>MAEIPKEMLRAQTNAILLNVLKQGDNYVYGIIKQVKEASNGEMELNEATLYTIFKRLEKDGIISSYWGDESQGGRRKYYRLTEIGHENMRLAFESWSRVDKIIENLEANKKSEAIKSRWSHPQFEK[2x]

We present a new class of ArMs featuring a genetically encoded noble‐metal‐binding site based on a non‐canonical thiophenol‐based amino acid, 4‐mercaptophenylalanine (pSHF), incorporated in the transcriptional regulator LmrR through stop codon suppression. Next, we investigated the incorporation of pSHF into Lactococcal multidrug resistance regulator (LmrR), which has been demonstrated to be a highly versatile protein scaffold for artificial enzyme design. We selected position V15 for incorporation, since this places pSHF inside the hydrophobic pocket at the dimer interface. Here, we report a new class of artificial metalloenzymes featuring a genetically encoded thiophenol for binding noble metals and the application of this design approach by the creation of an artificial gold enzyme that shows efficient catalysis of abiological hydroamination reactions.

After establishing the incorporation and position of the pSHF residues in LmrR using X‐ray crystallography, we aimed to establish the binding mode of the gold ions in LmrR_V15pSHF−Au. An X‐ray crystal structure at 2.50 Å resolution was obtained via co‐crystallisation with KAuCN2, which is more water‐soluble than Au(SMe2)Cl and has been used extensively for heavy atom phasing in protein X‐ray crystallography. The crystal structure and crystallographic Fourier maps revealed the presence of one gold ion, coordinating one of the two pSHF residues in the LmrR_V15pSHF dimer (Supporting Information section 9). The gold atom is associated with a strong peak in the anomalous difference Fourier map, unambiguously establishing its identity and position in the crystal structure. In addition to the sulphur of the pSHF residue, a hydroxyl ion or water molecule appears to serve as a coordinating ligand of the gold ion, establishing a linear two‐coordination arrangement that is typical for Au(I). The gold atom is surrounded by the side chains of Asn19, Lys22, Phe93, and Met89 at a minimal distance of 4–5 Å, establishing a second coordination sphere and restricting the solvent accessibility of the gold. No clear anomalous difference peak is present near the other pSHF residue, and the electron density of this residue appears distorted and weak compared to its counterpart in the dimer, indicative of substantial conformational disorder. Although it is possible that gold is also bound to this second pSHF residue, contributing to the observed disorder, the X‐ray data is insufficient to determine this conclusively. Aggregate formation of LmrR_V15pSHF−Au is avoided because the two thiophenolic residues are spatially separated in the protein dimer. Of these, we selected two positions for site‐saturation mutagenesis: A11, which showed a faster reaction upon substitution to leucine, and M89, which in the crystal structure is in close proximity of the pSHF‐bound gold centre and gave rise to lower activity when replaced with alanine.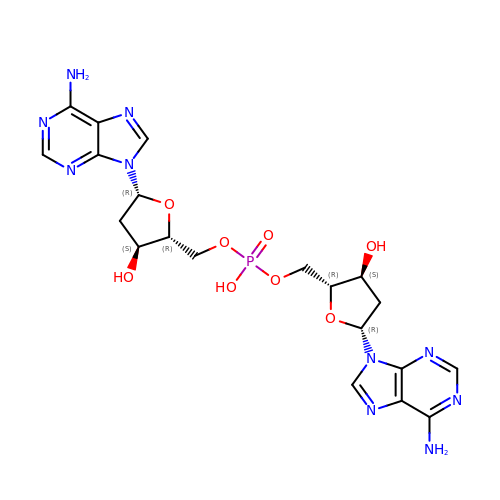bis{[(2R,3S,5R)-5-(6-amino-9H-purin-9-yl)-3-hydroxytetrahydrofuran-2-yl]methyl} hydrogen phosphate | C20 H25 N10 O8 P | PPQXTUORNPDZDR-PRSXHHODSA-N The MCM motor of the eukaryotic replicative helicase is loaded as a double hexamer onto DNA by the Origin Recognition Complex (ORC), Cdc6, and Cdt1. ATP binding supports formation of the ORC-Cdc6-Cdt1-MCM (OCCM) helicase-recruitment complex where ORC-Cdc6 and one MCM hexamer form two juxtaposed rings around duplex DNA. MCM is a ring-shaped helicase containing six related AAA+ ATPase polypeptides featuring bipartite active sites with catalytic residues contributed by neighbouring subunits. Biochemical studies established that ATP hydrolysis by MCM, but not ORC or Cdc6, are essential to complete helicase loading.

To further understand the role of ATP hydrolysis in OCCM-to-SH transition, we assembled a DH loading reaction using MCM-Cdt1 bearing the Mcm5RA variant. 3D classification identified two distinct states of a complex containing ORC-Cdt1-MCM but lacking Cdc6 (OC1MMcm5RA). While all ORC subunits are visible, the two states differ in the configuration of Orc1. In conformer 2, solved to 3.4 Å resolution in the consensus structure (or 3.3 and 3.5 Å when locally refining ORC and MCM-Cdt1, respectively), only the WHD but not the ATPase domain of Orc1 is visible. As a result, only two ATP molecules could be built in the ORC complex (at the Orc5-Orc4 and Orc3-Orc5 interfaces). One new contact is formed by Mcm5 WHD (unstructured in OCCMMcm2RA) that engages Orc3 WHD. One contact is lost, with Mcm7 WHD, which touches the Orc1 ATPase in OCCMMcm2RA and ATPγS-OCCM22, becoming disordered in OC1MMcm5RA. Compared to the OCCMMcm2RA, which contains a three-subunit ATPase spiral, the Mcm5 subunit engages Mcm2 in OC1MMcm5RA, capping the N-terminal end of a four-subunit spiral. Nucleotide (ADP, according to the cryo-EM density) can be observed bound to each of the Mcm4-6-2-5 subunits forming the ATPase spiral, but not to the Mcm3 and Mcm7 subunits. As observed for all other DNA-bound MCM subunits, the Mcm5 PS1 hairpin selectively engages the leading strand downstream of Mcm2 and the h2i hairpin predominantly binds the lagging strand.

> MSDNRRRRREEDDSDSENELPPSSPQQHFRGGMNPVSSPIGSPDMINPEGDDNEVDDVPDIDEVEEQMNEVDLMDDNMYEDYAADHNRDRYDPDQVDDREQQELSLSERRRIDAQLNERDRLLRNVAYIDDEDEEQEGAAQLDEMGLPVQRRRRRRQYEDLENSDDDLLSDMDIDPLREELTLESLSNVKANSYSEWITQPNVSRTIARELKSFLLEYTDETGRSVYGARIRTLGEMNSESLEVNYRHLAESKAILALFLAKCPEEMLKIFDLVAMEATELHYPDYARIHSEIHVRISDFPTIYSLRELRESNLSSLVRVTGVVTRRTGVFPQLKYVKFNCLKCGSILGPFFQDSNEEIRISFCTNCKSKGPFRVNGEKTVYRNYQRVTLQEAPGTVPPGRLPRHREVILLADLVDVSKPGEEVEVTGIYKNNYDGNLNAKNGFPVFATIIEANSIKRREGNTANEGEEGLDVFSWTEEEEREFRKISRDRGIIDKIISSMAPSIYGHRDIKTAVACSLFGGVPKNVNGKHSIRGDINVLLLGDPGTAKSQILKYVEKTAHRAVFATGQGASAVGLTASVRKDPITKEWTLEGGALVLADKGVCLIDEFDKMNDQDRTSIHEAMEQQSISISKAGIVTTLQARCSIIAAANPNGGRYNSTLPLAQNVSLTEPILSRFDILCVVRDLVDEEADERLATFVVDSHVRSHPENDEDREGEELKNNGESAIEQGEDEINEQLNARQRRLQRQRKKEEEISPIPQELLMKYIHYARTKIYPKLHQMDMDKVSRVYADLRRESISTGSFPITVRHLESILRIAESFAKMRLSEFVSSYDLDRAIKVVVDSFVDAQKVSVRRQLRRSFAIYTLGH;> MKRRWKKNFIAVSAANRFKKISSSGALENLYFQGEMEGSTGFDGDATTFFAPDAVFGDRVRRFQEFLDTFTSYRDSVRSIQVYNSNNAANYNDDQDDADERDLLGDDDGDDLEKEKKAASSTSLNILPHRIIISLDDLREFDRSFWSGILVEPAYFIPPAEKALTDLADSMDDVPHPNASAVSSRHPWKLSFKGSFGAHALSPRTLTAQHLNKLVSVEGIVTKTSLVRPKLIRSVHYAAKTGRFHYRDYTDATTTLTTRIPTPAIYPTEDTEGNKLTTEYGYSTFIDHQRITVQEMPEMAPAGQLPRSIDVILDDDLVDKTKPGDRVNVVGVFKSLGAGGMNQSNSNTLIGFKTLILGNTVYPLHARSTGVAARQMLTDFDIRNINKLSKKKDIFDILSQSLAPSIYGHDHIKKAILLMLMGGVEKNLENGSHLRGDINILMVGDPSTAKSQLLRFVLNTASLAIATTGRGSSGVGLTAAVTTDRETGERRLEAGAMVLADRGVVCIDEFDKMTDVDRVAIHEVMEQQTVTIAKAGIHTTLNARCSVIAAANPVFGQYDVNRDPHQNIALPDSLLSRFDLLFVVTDDINEIRDRSISEHVLRTHRYLPPGYLEGEPVRERLNLSLAVGEDADINPEEHSNSGAGVENEGEDDEDHVFEKFNPLLQAGAKLAKNKGNYNGTEIPKLVTIPFLRKYVQYAKERVIPQLTQEAINVIVKNYTDLRNDDNTKKSPITARTLETLIRLATAHAKVRLSKTVNKVDAKVAANLLRFALLGEDIGNDIDEEESEYEEALSKRSPQKSPKKRQRVRQPASNSGSPIKSTPRRSTASSVNATPSSARRILRFQDDEQNAGEDDNDIMSPLPADEEAELQRRLQLGLRVSPRRREHLHAPEEGSSGPLTEVGTPRLPNVSSAGQDDEQQQSVISFDNVEPGTISTGRLSLISGIIARLMQTEIFEEESYPVASLFERINEELPEEEKFSAQEYLAGLKIMSDRNNLMVADDKVWRV;> MSQQSSSPTKEDNNSSSPVVPNPDSVPPQLSSPALFYSSSSSQGDIYGRNNSQNLSQGEGNIRAAIGSSPLNFPSSSQRQNSDVFQSQGRQGRIRSSASASGRSRYHSDLRSDRALPTSSSSLGRNGQNRVHMRRNDIHTSDLSSPRRIVDFDTRSGVNTLDTSSSSAPPSEASEPLRIIWGTNVSIQECTTNFRNFLMSFKYKFRKILDEREEFINNTTDEELYYIKQLNEMRELGTSNLNLDARNLLAYKQTEDLYHQLLNYPQEVISIMDQTIKDCMVSLIVDNNLDYDLDEIETKFYKVRPYNVGSCKGMRELNPNDIDKLINLKGLVLRSTPVIPDMKVAFFKCNVCDHTMAVEIDRGVIQEPARCERIDCNEPNSMSLIHNRCSFADKQVIKLQETPDFVPDGQTPHSISLCVYDELVDSCRAGDRIEVTGTFRSIPIRANSRQRVLKSLYKTYVDVVHVKKVSDKRLDVDTSTIEQELMQNKVDHNEVEEVRQITDQDLAKIREVAAREDLYSLLARSIAPSIYELEDVKKGILLQLFGGTNKTFTKGGRYRGDINILLCGDPSTSKSQILQYVHKITPRGVYTSGKGSSAVGLTAYITRDVDTKQLVLESGALVLSDGGVCCIDEFDKMSDSTRSVLHEVMEQQTISIAKAGIITTLNARSSILASANPIGSRYNPNLPVTENIDLPPPLLSRFDLVYLVLDKVDEKNDRELAKHLTNLYLEDKPEHISQDDVLPVEFLTMYISYAKEHIHPIITEAAKTELVRAYVGMRKMGDDSRSDEKRITATTRQLESMIRLAEAHAKMKLKNVVELEDVQEAVRLIRSAIKDYATDPKTGKIDMNLVQTGKSVIQRKLQEDLSREIMNVLKDQASDSMSFNELIKQINEHSQDRVESSDIQEALSRLQQEDKVIVLGEGVRRSVRLNNRV;> MSFDRPEIYSAPVLQGESPNDDDNTEIIKSFKNFILEFRLDSQFIYRDQLRNNILVKNYSLTVNMEHLIGYNEDIYKKLSDEPSDIIPLFETAITQVAKRISILSRAQSANNNDKDPENTSMDTDSLLLNSLPTFQLILNSNANQIPLRDLDSEHVSKIVRLSGIIISTSVLSSRATYLSIMCRNCRHTTSITINNFNSITGNTVSLPRSCLSTIESESSMANESNIGDESTKKNCGPDPYIIIHESSKFIDQQFLKLQEIPELVPVGEMPRNLTMTCDRYLTNKVIPGTRVTIVGIYSIYNSKNGAGSGRSGGGNGGSGVAIRTPYIKILGIQSDVETSSIWNSVTMFTEEEEEEFLQLSRNPKLYEILTNSIAPSIFGNEDIKKAIVCLLMGGSKKILPDGMRLRGDINVLLLGDPGTAKSQLLKFVEKVSPIAVYTSGKGSSAAGLTASVQRDPMTREFYLEGGAMVLADGGVVCIDEFDKMRDEDRVAIHEAMEQQTISIAKAGITTVLNSRTSVLAAANPIYGRYDDLKSPGDNIDFQTTILSAFDMIFIVKDDHNEERDISIANHVINIHTGNANAMQNQQEENGSEISIEKMKRYITYCRLKCAPRLSPQAAEKLSSNFVTIRKQLLINELESTERSSIPITIRQLEAIIRITESLAKLELSPIAQERHVDEAIRLFQASTMDAASQDPIGGLNQASGTSLSEIRRFEQELKRRLPIGWSTSYQTLRREFVDTHRFSQLALDKALYALEKHETIQLRHQGQNIYRSGV;> MSSPFPADTPSSNRPSNSSPPPSSIGAGFGSSSGLDSQIGSRLHFPSSSQPHVSNSQTGPFVNDSTQFSSQRLQTDGSATNDMEGNEPARSFKSRALNHVKKVDDVTGEKVREAFEQFLEDFSVQSTDTGEVEKVYRAQIEFMKIYDLNTIYIDYQHLSMRENGALAMAISEQYYRFLPFLQKGLRRVVRKYAPELLNTSDSLKRSEGDEGQADEDEQQDDDMNGSSLPRDSGSSAAPGNGTSAMATRSITTSTSPEQTERVFQISFFNLPTVHRIRDIRSEKIGSLLSISGTVTRTSEVRPELYKASFTCDMCRAIVDNVEQSFKYTEPTFCPNPSCENRAFWTLNVTRSRFLDWQKVRIQENANEIPTGSMPRTLDVILRGDSVERAKPGDRCKFTGVEIVVPDVTQLGLPGVKPSSTLDTRGISKTTEGLNSGVTGLRSLGVRDLTYKISFLACHVISIGSNIGASSPDANSNNRETELQMAANLQANNVYQDNERDQEVFLNSLSSDEINELKEMVKDEHIYDKLVRSIAPAVFGHEAVKKGILLQMLGGVHKSTVEGIKLRGDINICVVGDPSTSKSQFLKYVVGFAPRSVYTSGKASSAAGLTAAVVRDEEGGDYTIEAGALMLADNGICCIDEFDKMDISDQVAIHEAMEQQTISIAKAGIHATLNARTSILAAANPVGGRYNRKLSLRGNLNMTAPIMSRFDLFFVILDDCNEKIDTELASHIVDLHMKRDEAIEPPFSAEQLRRYIKYARTFKPILTKEARSYLVEKYKELRKDDAQGFSRSSYRITVRQLESMIRLSEAIARANCVDEITPSFIAEAYDLLRQSIIRVDVDDVEMDEEFDNIESQSHAASGNNDDNDDGTGSGVITSEPPADIEEGQSEATARPGTSEKKKTTVTYDKYVSMMNMIVRKIAEVDREGAEELTAVDIVDWYLLQKENDLGSLAEYWEERRLAFKVIKRLVKDRILMEIHGTRHNLRDLENEENENNKTVYVIHPNCEVLDQLEPQDSS;> MSAALPSIQLPVDYNNLFNEITDFLVTFKQDTLSSDATRNENEDENLDAENIEQHLLEKGPKYMAMLQKVANRELNSVIIDLDDILQYQNEKFLQGTQADDLVSAIQQNANHFTELFCRAIDNNMPLPTKEIDYKDDVLDVILNQRRLRNERMLSDRTNEIRSENLMDTTMDPPSSMNDALREVVEDETELFPPNLTRRYFLYFKPLSQNCARRYRKKAISSKPLSVRQIKGDFLGQLITVRGIITRVSDVKPAVEVIAYTCDQCGYEVFQEVNSRTFTPLSECTSEECSQNQTKGQLFMSTRASKFSAFQECKIQELSQQVPVGHIPRSLNIHVNGTLVRSLSPGDIVDVTGIFLPAPYTGFKALKAGLLTETYLEAQFVRQHKKKFASFSLTSDVEERVMELITSGDVYNRLAKSIAPEIYGNLDVKKALLLLLVGGVDKRVGDGMKIRGDINVCLMGDPGVAKSQLLKAICKISPRGVYTTGKGSSGVGLTAAVMKDPVTDEMILEGGALVLADNGICCIDEFDKMDESDRTAIHEVMEQQTISISKAGINTTLNARTSILAAANPLYGRYNPRLSPLDNINLPAALLSRFDILFLMLDIPSRDDDEKLAEHVTYVHMHNKQPDLDFTPVEPSKMREYIAYAKTKRPVMSEAVNDYVVQAYIRLRQDSKREMDSKFSFGQATPRTLLGIIRLSQALAKLRLADMVDIDDVEEALRLVRVSKESLYQETNKSKEDESPTTKIFTIIKKMLQETGKNTLSYENIVKTVRLRGFTMLQLSNCIQEYSYLNVWHLINEGNTLKFVDDGTMDTDQEDSLVSTPKLAPQTTASANVSAQDSDIDLQDA;> MSGTANSRRKEVLRVPVIDLNRVSDEEQLLPVVRAILLQHDTFLLKNYANKAVLDALLAGLTTKDLPDTSQGFDANFTGTLPLEDDVWLEQYIFDTDPQLRFDRKCRNESLCSIYSRLFKLGLFFAQLCVKSVVSSAELQDCISTSHYATKLTRYFNDNGSTHDGADAGATVLPTGDDFQYLFERDYVTFLPTGVLTIFPCAKAIRYKPSTMATTDNSWVSIDEPDCLLFHTGTLLARWSQGMHTTSPLQIDPRANIVSLTIWPPLTTPISSKGEGTIANHLLEQQIKAFPKVAQQYYPRELSILRLQDAMKFVKELFTVCETVLSLNALSRSTGVPPELHVLLPQISSMMKRKIVQDDILKLLTIWSDAYVVELNSRGELTMNLPKRDNLTTLTNKSRTLAFVERAESWYQQVIASKDEIMTDVPAFKINKRRSSSNSKTVLSSKVQTKSSNANALNNSRYLANSKENFMYKEKMPDSQANLMDRLRERERRSAALLSQRQKRYQQFLAMKMTQVFDILFSLTRGQPYTETYLSSLIVDSLQDSNNPIGTKEASEILAGLQGILPMDISVHQVDGGLKVYRWNSLDKNRFSKLLQIHKSKQQD;> MKRRWKKNFIAVSAANRFKKISSSGALENLYFQGEMAKTLKDLQGWEIITTDEQGNIIDGGQKRLRRRGAKTEHYLKRSSDGIKLGRGDSVVMHNEAAGTYSVYMIQELRLNTLNNVVELWALTYLRWFEVNPLAHYRQFNPDANILNRPLNYYNKLFSETANKNELYLTAELAELQLFNFIRVANVMDGSKWEVLKGNVDPERDFTVRYICEPTGEKFVDINIEDVKAYIKKVEPREAQEYLKDLTLPSKKKEIKRGPQKKDKATQTAQISDAETRATDITDNEDGNEDESSDYESPSDIDVSEDMDSGEISADELEEEEDEEEDEDEEEKEARHTNSPRKRGRKIKLGKDDIDASVQPPPKKRGRKPKDPSKPRQMLLISSCRANNTPVIRKFTKKNVARAKKKYTPFSKRFKSIAAIPDLTSLPEFYGNSSELMASRFENKLKTTQKHQIVETIFSKVKKQLNSSYVKEEILKSANFQDYLPARENEFASIYLSAYSAIESDSATTIYVAGTPGVGKTLTVREVVKELLSSSAQREIPDFLYVEINGLKMVKPTDCYETLWNKVSGERLTWAASMESLEFYFKRVPKNKKKTIVVLLDELDAMVTKSQDIMYNFFNWTTYENAKLIVIAVANTMDLPERQLGNKITSRIGFTRIMFTGYTHEELKNIIDLRLKGLNDSFFYVDTKTGNAILIDAAGNDTTVKQTLPEDVRKVRLRMSADAIEIASRKVASVSGDARRALKVCKRAAEIAEKHYMAKHGYGYDGKTVIEDENEEQIYDDEDKDLIESNKAKDDNDDDDDNDGVQTVHITHVMKALNETLNSHVITFMTRLSFTAKLFIYALLNLMKKNGSQEQELGDIVDEIKLLIEVNGSNKFVMEIAKTLFQQGSDNISEQLRIISWDFVLNQLLDAGILFKQTMKNDRICCVKLNISVEEAKRAMNEDETLRNL;> MLNGEDFVEHNDILSSPAKSRNVTPKRVDPHGERQLRRIHSSKKNLLERISLVGNERKNTSPDPALKPKTPSKAPRKRGRPRKIQEELTDRIKKDEKDTISSKKKRKLDKDTSGNVNEESKTSNNKQVMEKTGIKEKREREKIQVATTTYEDNVTPQTDDNFVSNSPEPPEPATPSKKSLTTNHDFTSPLKQIIMNNLKEYKDSTSPGKLTLSRNFTPTPVPKNKKLYQTSETKSASSFLDTFEGYFDQRKIVRTNAKSRHTMSMAPDVTREEFSLVSNFFNENFQKRPRQKLFEIQKKMFPQYWFELTQGFSLLFYGVGSKRNFLEEFAIDYLSPKIAYSQLAYENELQQNKPVNSIPCLILNGYNPSCNYRDVFKEITDLLVPAELTRSETKYWGNHVILQIQKMIDFYKNQPLDIKLILVVHNLDGPSIRKNTFQTMLSFLSVIRQIAIVASTDHIYAPLLWDNMKAQNYNFVFHDISNFEPSTVESTFQDVMKMGKSDTSSGAEGAKYVLQSLTVNSKKMYKLLIETQMQNMGNLSANTGPKRGTQRTGVELKLFNHLCAADFIASNEIALRSMLREFIEHKMANITKNNSGMEIIWVPYTYAELEKLLKTVLNTL;> MSDLNQSKKMNVSEFADAQRSHYTVYPSLPQSNKNDKHIPFVKLLSGKESEVNVEKRWELYHQLHSHFHDQVDHIIDNIEADLKAEISDLLYSETTQKRRCFNTIFLLGSDSTTKIELKDESSRYNVLIELTPKESPNVRMMLRRSMYKLYSAADAEEHPTIKYEDINDEDGDFTEQNNDVSYDLSLVENFKRLFGKDLAMVFNFKDVDSINFNTLDNFIILLKSAFKYDHVKISLIFNINTNLSNIEKNLRQSTIRLLKRNYHKLDVSSNKGFKYGNQIFQSFLDTVDGKLNLSDRFVEFILSKMANNTNHNLQLLTKMLDYSLMSYFFQNAFSVFIDPVNVDFLNDDYLKILSRCPTFMFFVEGLIKQHAPADEILSLLTNKNRGLEEFFVEFLVRENPINGHAKFVARFLEEELNITNFNLIELYHNLLIGKLDSYLDRWSACKEYKDRLHFEPIDTIFQELFTLDNRSGLLTQSIFPSYKSNIEDNLLSWEQVLPSLDKENYDTLSGDLDKIMAPVLGQLFKLYREANMTINIYDFYIAFRETLPKEEILNFIRKDPSNTKLLELAETPDAFDKVALILFMQAIFAFENMGLIKFQSTKSYDLVEKCVWRGI;> MTISEARLSPQVNLLPIKRHSNEEVEETAAILKKRTIDNEKCKDSDPGFGSLQRRLLQQLYGTLPTDEKIIFTYLQDCQQEIDRIIKQSIIQKESHSVILVGPRQSYKTYLLDYELSLLQQSYKEQFITIRLNGFIHSEQTAINGIATQLEQQLQKIHGSEEKIDDTSLETISSGSLTEVFEKILLLLDSTTKTRNEDSGEVDRESITKITVVFIFDEIDTFAGPVRQTLLYNLFDMVEHSRVPVCIFGCTTKLNILEYLEKRVKSRFSQRVIYMPQIQNLDDMVDAVRNLLTVRSEISPWVSQWNETLEKELSDPRSNLNRHIRMNFETFRSLPTLKNSIIPLVATSKNFGSLCTAIKSCSFLDIYNKNQLSNNLTGRLQSLSDLELAILISAARVALRAKDGSFNFNLAYAEYEKMIKAINSRIPTVAPTTNVGTGQSTFSIDNTIKLWLKKDVKNVWENLVQLDFFTEKSAVGLRDNATAAFYASNYQFQGTMIPFDLRSYQMQIILQELRRIIPKSNMYYSWTQL;> MNVTTPEVAFREYQTNCLASYISADPDITPSNLILQGYSGTGKTYTLKKYFNANPNLHAVWLEPVELVSWKPLLQAIARTVQYKLKTLYPNIPTTDYDPLQVEEPFLLVKTLHNIFVQYESLQEKTCLFLILDGFDSLQDLDAALFNKYIKLNELLPKDSKINIKFIYTMLETSFLQRYSTHCIPTVMFPRYNVDEVSTILVMSRCGELMEDSCLRKRIIEEQITDCTDDQFQNVAANFIHLIVQAFHSYTGNDIFALNDLIDFKWPKYVSRITKENIFEPLALYKSAIKLFLSTDDNLSENGQGESAITTNRDDLENSQTYDLSIISKYLLIASYICSYLEPRYDASIFSRKTRIIQGRAAYGRRKKKEVNPRYLQPSLFAIERLLAIFQAIFPIQGKAESGSLSALREESLMKANIEVFQNLSELHTLKLIATTMNKNIDYLSPKVRWKVNVPWEIIKEISESVHFNISDYFSDIHE;> MSMQQVQHCVAEVLRLDPQEKPDWSSGYLKKLTNATSILYNTSLNKVMLKQDEEVARCHICAYIASQKMNEKHMPDLCYYIDSIPLEPKKAKHLMNLFRQSLSNSSPMKQFAWTPSPKKNKRSPVKNGGRFTSSDPKELRNQLFGTPTKVRKSQNNDSFVIPELPPMQTNESPSITRRKLAFEEDEDEDEEEPGNDGLSLKSHSNKSITGTRNVDSDEYENHESDPTSEEEPLGVQESRSGRTKQNKAVGKPQSELKTAKALRKRGRIPNSLLVKKYCKMTTEEIIRLCNDFELPREVAYKIVDEYNINASRLVCPWQLVCGLVLNCTFIVFNERRRKDPRIDHFIVSKMCSLMLTSKVDDVIECVKLVKELIIGEKWFRDLQIRYDDFDGIRYDEIIFRKLGSMLQTTNILVTDDQYNIWKKRIEMDLALTEPL>[6x]MIPVTELRYFADTQPAYRILKPWWDVFTDYISIVMLMIAVFGGTLQVTQDKMICLPCKWVTKDSCNDSFRGWAAPGPEPTYPNSTILPTPDTGPTGIKYDLDRHQYNYVDAVCYENRLHWFAKYFPYLVLLHTLIFLACSNFWFKFPRTSSKLEHFVSILLKCFDSPWTTRALSETVVEESDPKPAFSKMNGSMDKKSSTVSEDVEATVPMLQRTKSRIEQGIVDRSETGVLDKKEGEQAKALFEKVKKFRTHVEEGDIVYRLYMRQTIIKVIKFILIICYTVYYVHNIKFDVDCTVDIESLTGYRTYRCAHPLATLFKILASFYISLVIFYGLICMYTLWWMLRRSLKKYSFESIREESSYSDIPDVKNDFAFMLHLIDQYDPLYSKRFAVFLSEVSENKLRQLNLNNEWTLDKLRQRLTKNAQDKLELHLFMLSGIPDTVFDLVELEVLKLELIPDVTIPPSIAQLTGLKELWL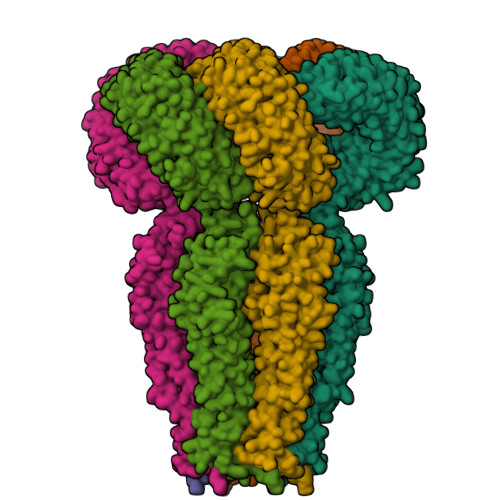YHTAAKIEAPALAFLRENLRALHIKFTDIKEIPLWIYSLKTLEELHLTGNLSAENNRYIVIDGLRELKRLKVLRLKSNLSKLPQVVTDVGVHLQKLSINNEGTKLIVLNSLKKMANLTELELIRCDLERIPHSIFSLHNLQEIDLKDNNLKTIEEIISFQHLHRLTCLKLWYNHIAYIPIQIGNLTNLERLYLNRNKIEKIPTQLFYCRKLRYLDLSHNNLTFLPADIGLLQNLQNLAITANRIETLPPELFQCRKLRALHLGNNVLQSLPSRVGELTNLTQIELRGNRLECLPVELGECPLLKRSGLVVEEDLFNTLPPEVKERLWRADKEQAGTENLYFQ> MSALPEEVNRTLLQIVQAFASPDNQIRSVAEKALSEEWITENNIEYLLTFLAEQAAFSQDTTVAALSAVLFRKLALKAPITHIRKEVLAQIRSSLLKGFLSERADSIRHKLSDAIAECVQDDLPAWPELLQALIESLKSGNPNFRESSFRILTTVPYLITAVDINSILPIFQSGFTDASDNVKIAAVTAFVGYFKQLPKSEWSKLGILLPSLLNSLPRFLDDGKDDALASVFESLIELVELAPKLFKDMFDQIIQFTDMVIKNKDLEPPARTTALELLTVFSENAPQMCKSNQNYGQTLVMVTLIMMTEVSIDDDDAAEWIESDDTDDEEEVTYDHARQALDRVALKLGGEYLAAPLFQYLQQMITS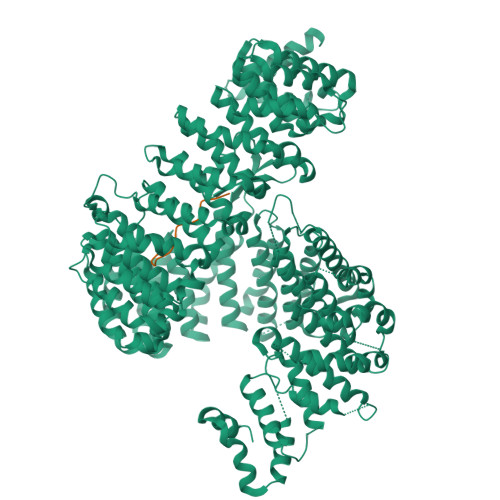TEWRERFAAMMALSSAAEGCADVLIGEIPKILDMVIPLINDPHPRVQYGCCNVLGQISTDFSPFIQRTAHDRILPALISKLTSECTSRVQTHAAAALVNFSEFASKDILEPYLDSLLTNLLVLLQSNKLYVQEQALTTIAFIAEAAKNKFIKYYDTLMPLLLNVLKVNNKDNSVLKGKCMECATLIGFAVGKEKFHEHSQELISILVALQNSDIDEDDALRSYLEQSWSRICRILGDDFVPLLPIVIPPLLITAKATQDVGLIEEEEAANFQQYPDWDVVQVQGKHIAIHTSVLDDKVSAMELLQSYATLLRGQFAVYVKEVMEEIALPSLDFYLHDGVRAAGATLIPILLSCLLAATGTQNEELVLLWHKASSKLIGGLMSEPMPEITQVYHNSLVNGIKVMGDNCLSEDQLAAFTKGVSANLTDTYERMQDRHGDGDEYNENIDEEEDFTDEDLLDEINKSIAAVLKTTNGHYLKNLENIWPMINTFLLDNEPILVIFALVVIGDLIQYGGEQTASMKNAFIPKVTECLISPDARIRQAASYIIGVCAQYAPSTYADVCIPTLDTLVQIVDFPGSKLEENRSSTENASAAIAKILYAYNSNIPNVDTYTANWFKTLPTITDKEAASFNYQFLSQLIENNSPIVCAQSNISAVVDSVIQALNERSLTEREGQTVISSVKKLLGFLPSSDAMAIFNRYPADIMEKVHKWFA;> PRRRTVGMKSSQGNVPTGNKQSVGKSAKISKPLHIKTSAYQKQYKINLETKARPSAGDEDSAHPDKNKE Human SIDT1 and SIDT2 are closely related members of the SID-1 transmembrane family, and have been implicated in various biological processes such as glucose and lipid metabolism, innate immunity, and tumorigenesis. Here, we present the cryo-electron microscopy (cryo-EM) structures of human SIDT1 and SIDT2. Both structures reveal an overall architecture of a dimeric arrangement composed of an extracellular domain (ECD) rich in β-strands and a transmembrane domain (TMD) with 11 passes, highlighting the remarkable structural congruence. Importantly, the ECDs of SIDT1 and SIDT2 bind synthetic plant-derived miRNA only under acidic conditions.

The TMDs of both proteins consist of 11 transmembrane helices and feature two pairs of conserved disulfide bonds that are essential for structural integrity. Notably, both SIDT1 and SIDT2 exhibit a potential zinc-binding site with three histidine residues within TMDs, which is responsible for lipid hydrolytic activity. Regarding the TMD, while the overall arrangement is similar in both SIDT1 and SIDT2, different transmembrane helices (TMs) contribute to dimerization. In SIDT1, the dimer interface primarily involves TM2 interacting with TM5 from the other protomer and is driven by extensive hydrophobic interactions. TM6 does not appear to play a significant role in the SIDT1 dimer interface. The electron density maps exhibited well-defined main-chain connectivity and side-chain densities in the ECDs, while the TMDs have relatively lower quality and resolution. The truncated TMD proteins also exhibited GFP fluorescence, suggesting that the TMD alone is sufficient for dimerization or oligomerization.

>[2x]IKESVYVKSSLFSVFIFLSFYLGCLLVGFVHYLRFQRKSIDGSFGSNDGSGNMVASHPIAASTPEPDIESDKNIIRTKMFLYLSDLSRKDRRIVSKKYKIYFWNIITIAVFYALPVIQLVITYQTVVNVTGNQDICYYNFLCAHPLGVLSAFNNILSNLGHVLLGFLFLLIVLRRDILHRRALEAKDIFAVEYGIPKHFGLFYAMGIALMMEGVLSACYHVCPNYSNFQFDTSFMYMIAGLCMLKLYQTRHPDINASAYSAYASFAVVIMVTVLGVVFGKNDVWFWVIFSAIHVLASLALSTQIYYMGRFKIDLGIFRRAAMVFYTDCIQQCSRPLYMDRMVLLVVGNLVNWSFALFGLIYRPRDFASYMLGIFICNLLLYLAFYIIMKLRSSEKVLPVPLFCIVATAVMWAAALYFFFQNLSSWEGTPAESREKNRECILLDFFDDHDIWHFLSATALFFSFLVLLTLDDDLDVVRRDQIPVFDYKDHDGDYKDHDIDYKDDDDK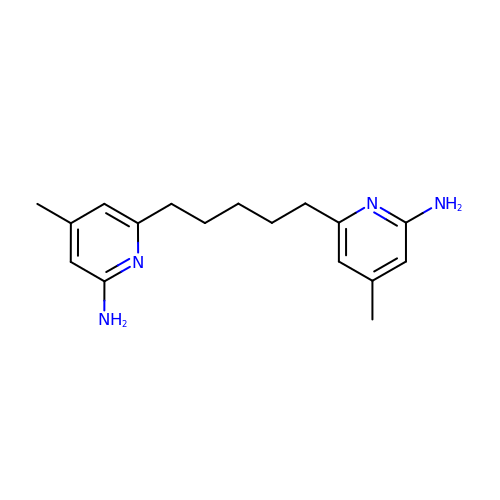6,6'-pentane-1,5-diylbis(4-methylpyridin-2-amine) | C17 H24 N4 | UWCJUMUVUHRQQV-UHFFFAOYSA-N>[4x]MVQASGHRRSTRGSKMVSWSVIAKIQEILQRKMVREFLAEFMSTYVMMVFGLGSVAHMVLNKKYGSYLGVNLGFGFGVTMGVHVAGRISGAHMNAAVTFANCALGRVPWRKFPVYVLGQFLGSFLAAATIYSLFYTAILHFSGGQLMVTGPVATA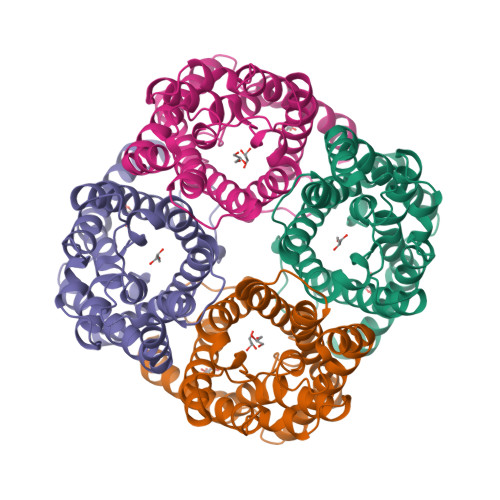GIFATYLPDHMTLWRGFLNEAWLTGMLQLCLFAITDQENNPALPGTEALVIGILVVIIGVSLGMNTGYAINPSRDLPPRIFTFIAGWGKQVFSNGENWWWVPVVAPLLGAYLGGIIYLVFIGSTIPREPLKLEDSVAYEDHGITVLPKMGSHEPTISPLTPVSVSPANRSSVHPAPPLHESMALEHFGGSLEVLFQGPAAYPYDVPDYAAAHHHHHHHHHH> MRERPHTSGHHGAGEARATAPSTVSPYGPEARAELSSRLTTLRNTLAPATNDPRYLQACGGEKLNRFRDIQCRRQTAVRADLNANYIQVGNTRTIACQYPLQSQLESHFRMLAENRTPVLAVLASSSEIANQRFGMPDYFRQSGTYGSITVESKMTQQVGLGDGIMADMYTLTIREAGQKTI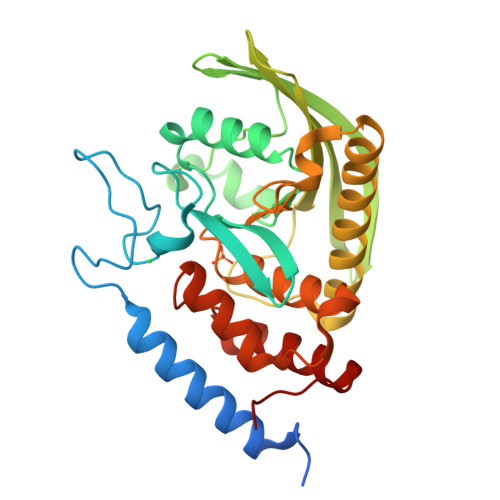SVPVVHVGNWPDQTAVSSEVTKALASLVDQTAETKRNMYESKGSSAVADDSKLRPVIHSRAGVGRTAQLIGAMCMNDSRNSQLSVEDMVSQMRVQRNGIMVQKDEQLDVLIKLAEGQGRPLLNS>MELIRIAMKKDLENDNSLMNKWATVAGLKNPNPLYDFLNHDGKTFNEFSSIVNIVKSQYPDREYELMKDYCLNLDVKTKAARSALEYADANMFFEIEDVLIDSMISCSNMKSKEYGKVYKIHRELSNSVITEFEAVKRLGKLNIKTPEMNSFSRLLLLYHYLSTGNFSPMAQLIKQIDLSEISENMYIRNTYQTRVHVLMSNIKLNENSLEECREYSKKALESTNILRFQVFSYLTIGNSLLFSNYELAQENFLKGLSISVQNENYNMIFQQALCFLNNVWRKENKWINFESDSIMDLQEQAHCFINFNEN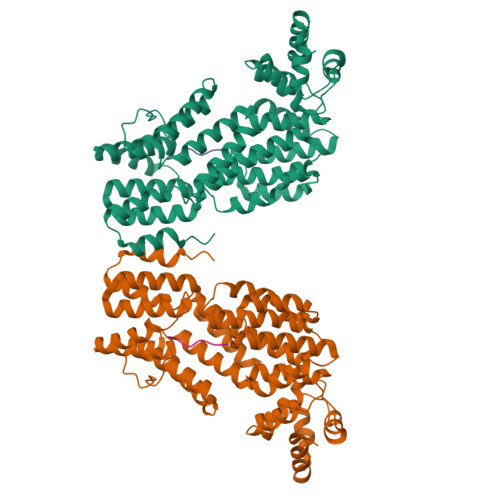SKAKEVLDKLDLLVHNDNELAMHYYLKGRLEQNKACFYSSIEYFKKSNDKFLIRLPLLELQKMGENQKLLELLLLLEHHH[2x];>GMPRGA[2x]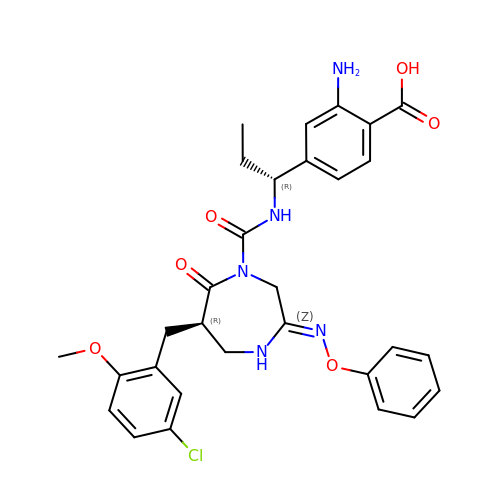2-amino-4-((R)-1-((R,Z)-6-(5-chloro-2-methoxybenzyl)-7-oxo-3-(phenoxyimino)-1,4-diazepane-1-carboxamido)propyl)benzoic acid | C30 H32 Cl N5 O6 | LHASZEBEQGPCFM-CJFMBICVSA-N> DYKDDDAMGTKLEDSPPCRNWSSASELNETQEPFLNPTDYDDEEFLRYLWREYLHPKEYEWVLIAGYIIVFVVALIGNVLVCVAVWKNHHMRTVTNYFIVNLSLADVLVTITCLPATLVVDITETWFFGQSLCKVIPYLQTVSVSVSVLTLSCIALDRWYAICHPLMFKSTAKRARNSIVIIWIVSCIIMIPQAIVMECSTVFPGLANKTTLFTVCDERWGGEIYPKMYHICFFLVTYMAPLCLMVLAYLQIFRKLWCRQGIDCSFWNESYLTGSRDERKKSLLSKFGMDEGVTFMFIGRFDRGQKGVDVLLKAIEILSSKKEFQEMRFIIIGKGDPELEGWARSLEEKHGNVKVITEMLSREFVRELYGSVDFVIIPSYFEPFGLVALEAMCLGAIPIASAVGGLRDIITNETGILVKAGDPGELANAILKALELSRSDLSKFRENCKKRAMSFSKQIRARRKTARMLMVVLLVFAICYLPISILNVLKRVFGMFAHTEDRETVYAWFTFSHWLVYANSAANPIIYNFLSGKFREE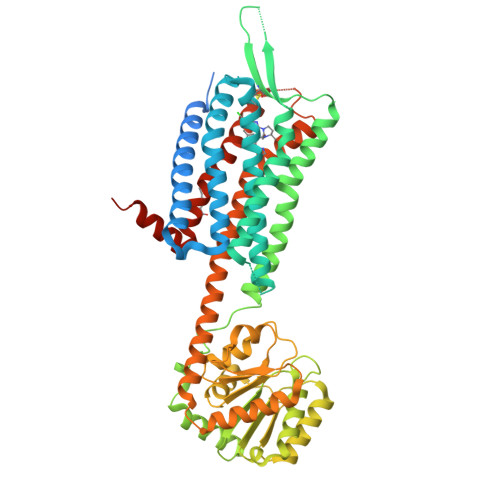FKAAFSCCCLGVHHHHHHHHHH>[14x]GSHMKDKDLLKGLDQEQANEVIAVLQMHNIEANKIDSGKLGYSI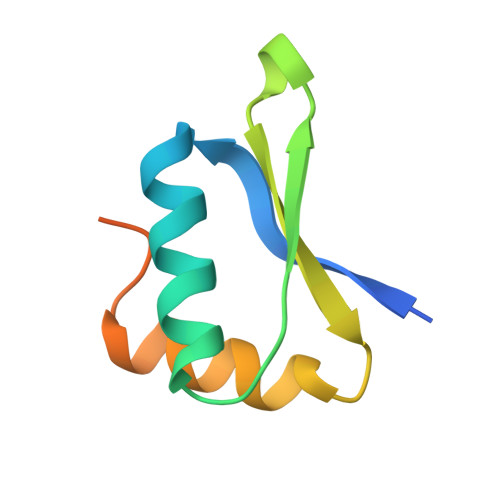TVAEPDFTAAVYWIKTYQLPPRPRVEIAQMFPAD>[4x]MTPKPKIVLVGSGMIGGVMATLIVQKNLGDVVMFDVVKNMPQGKALDTSHSNVMAYSNCKVTGSNSYDDLKGADVVIVTAGFTKAPGKSDKEWNRDDLLPLNNKIMIEIGGHIKNLCPNAFIIVVTNPVDVMVQLLFEHSGVPKNKIIGLGGVLDTSRLKYYISQKLNVCPRDVNALIVG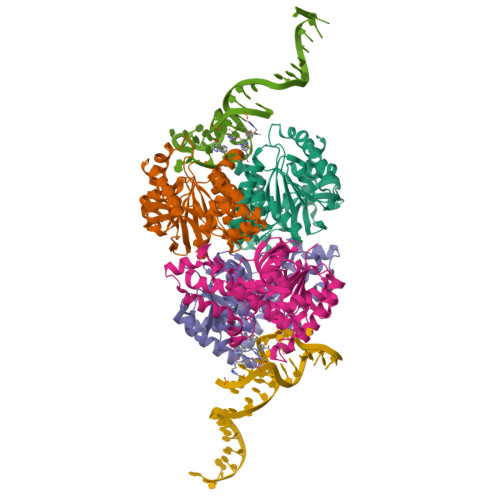AHGNKMVLLKRYITVGGIPLQEFINNKKITDEEVEGIFDRTVNTALEIVNLLASPYVAPAAAIIEMAESYLKDIKKVLVCSTLLEGQYGHSNIFGGTPLVIGGTGVEQVIELQLNAEEKTKFDEAVAETKRMKALI> HMPLRRPAHRGDGMTRPPAPPPGAPGADELLDCGLLSPVRAGTPVEALVCDSAWLQAMLDAEAALTRAQARTGFLPAAAAEAITAAARADRIDLLAVARGARETANPVVGLVAALTAAVRRDDPAAAEYVHRGSTSQDVLDTGAMLVARRALRLIGDDLDRAADALAALAADHRDTPMAGRTLALHAVPTTFGLKAAGWLELVSEAAGRVARLRDGLPFSLGGAAGTLAGYFGDRTDRGDPAVLLDRLLDAYAAETGLARPVLPWHVLRTPVADLAAVLAFTAGALGKIAVDVQSLARTEVAEVAEPAVEGRGASSAMPHKRNPVLSTLIRSAALQVPALATGLTQCLVSEDERSAGAWHAEWQPLRECLRLTGGAARTAVELAAGLEVDAARMRANLDLTDGRIVSESVAVALTPLLGRQAAKELLTRAAFTAGHEGRTLGEVLGELPELDGVLPKERWEALLDPARATGVAGALVDGA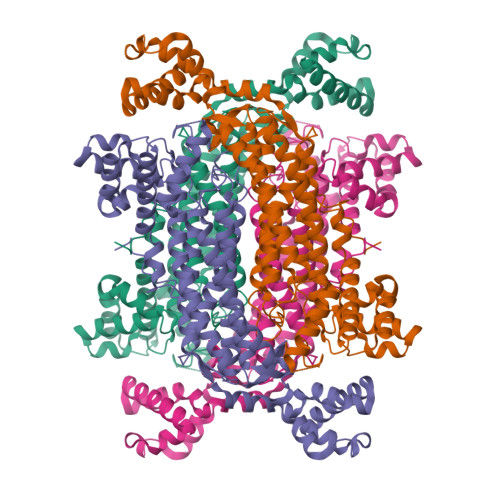LARRRPPAR>[2x]SNANDIRSKKVLIIGAGSLGSMIAENLMRIGVVSQGILDADLLQTGNLSRHALTMTSVGHNKAAALVEHLNRILPDASARSFSCAFPPESEVAKN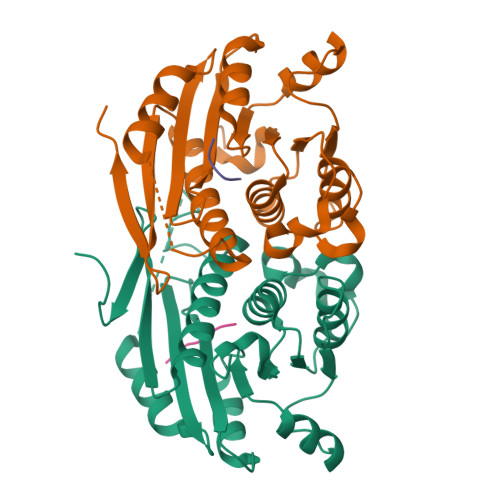SLRQYDVIIDCTGDDGVLKSLAAFDWKSEKIFISLAMTWRAEGLFAFAASETSFPVTDASSRFNASASPEIDMDEARIEGIGAWHPVFPARADDVQLWAAVGTKFICRVVSAPGRIYEYFKQMPDGTVEKEPHEYGSG;>[2x]KPAEPQKTGRFA>MGVEDEPLLRENPRRFVIFPIEYHDIWQMYKKAEASFWTAEEVDLSKDIQHWE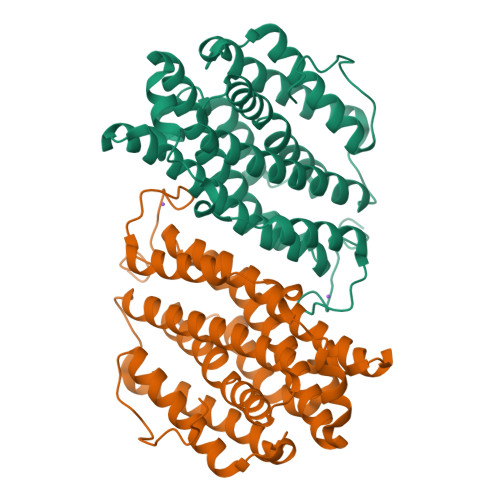SLKPEERYFISHVLAFFAASDGIVNENLVERFSQEVQITEARCFYGFQIAMENIHSEMYSLLIDTYIKDPKEREFLFNAIETMPCVKKKADWALRWIGDKEATYGERVVAFAAVEGIFFSGSFASIFWLKKRGLMPGLTFSNELISRDEGLHCDFACLMFKHLVHKPSEERVREIIINAVRIEQEFLTEALPVKLIGMNCTLMKQYIEFVADRLMLELGFSKVFRVENPFDFM[4x]>HQSQLDRERILSLEQRVVELQQTLAQKDQALGKLEQSLRLMEEASFDGTFLWKITNVTRRCHESACGRTVSLFSPAFYTAKYGYKLCLRLYLNGDGTGKRTHLSLFIVIMRG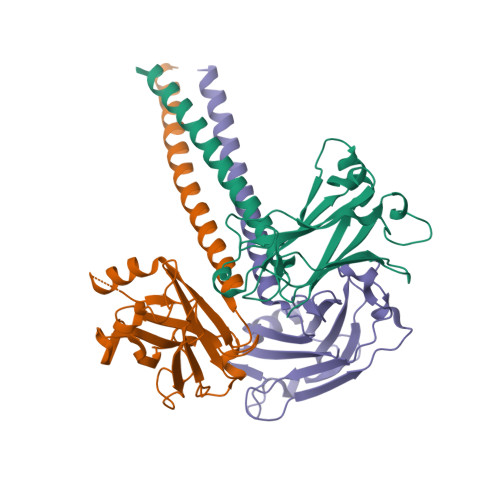EYDALLPWPFRNKVTFMLLDQNNREHAIDAFRPDLSSASFQRPQSETNVASGCPLFFPLSKLQSPKHAYVKDDTMFLKCIVETST[3x]> GPLGSLTMGAQDTLPVAAAFTETVNAYFKGADPSKCIVKITGEMVLSFPAGITRHFANNPSPAALTFRVINFSRLEHVLPNPQLLCCDNTQNDANTKEFWVNMPNLMTHLKKVSEQKPQATYYNVDMLKYQVSAQGIQSTPLNLAVNWRCEPSSTDLRIDYKYNTDAMTTAVALNNVQFLVPIDGGVTKLQAVLPPAVWNAEQQRILWKIPDISQKSENGGVGSLLARFQLSEGPSKPSPLVVQFTSEGSTLSGCDIELVGAGYRFSLI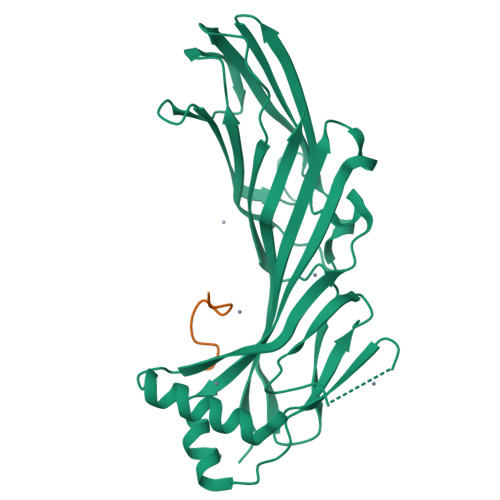KKRFAAGKYLADN;> YDPFGGDPFKG> SGTESGVSSRIIGGEQATAGEWPYMVALTARNSSHVFCGGSYLGGRYVLTAAHCVDKEDPAKGDVLLGAFDMNDVNTAERIHVRQIYVHNSYITASMGNDIAVLELERDPLPRRSVQISDSSDFNELTKDSPMTVIGFGNRKEVDGEKSDPATILHQVQVPFVPLPECKTKGSDQDAKNNYSQLTNNAFCAGSFGKDACSGDAGGPIFFDSNNGRKQMGVVSWGDGCGRANSPGVYTNLSVFNDWLDDQQLGLSYRQKRDLGVVRPGSYTHNLTFTNNGNADINLGNTFVFVVGISRTDAAAIVNNSCTGVLASGASCDVEFSYNITEHKQSYVKLIIGSSTYKTGAVHAYLYFDALDAAPSETVSFLANLPVHNTHVNDHPWTVVGNGLQTSALPAGEESVILLENLPQGRLKFHYKLSSSEVLDQLFVYVNDKFKGKYFNNTENLATLDMYGTNNKVRFVYRRHSGSTDDQSRAI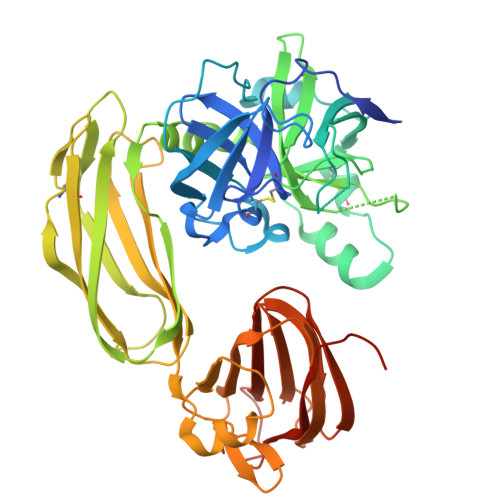LSQISYDPKFFDLPPPLDIRIGDENLYFQ> GPETLCGAELVDALQFVCGDRG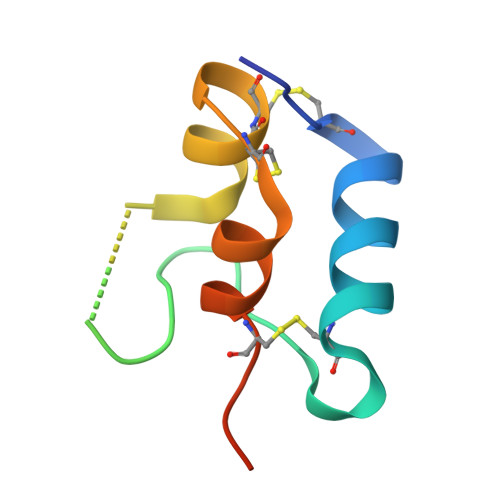FYFNKPTGYGSSSRRAPQTGIVDECCFRSCDLRRLEMYCAPLKPAKSA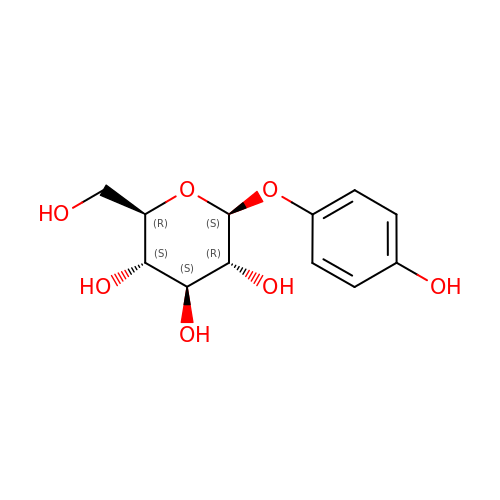(2R,3S,4S,5R,6S)-2-(hydroxymethyl)-6-(4-oxidanylphenoxy)oxane-3,4,5-triol | C12 H16 O7 | BJRNKVDFDLYUGJ-RMPHRYRLSA-N> MRSTQEERFEQRIAQETAIEPQDWMPDAYRKTLIRQIGQHAHSEIVGMLPEGNWITRAPTLRRKAILLAKVQDEAGHGLYLYSAAETLGCAREDIYQKMLDGRMKYSSIFNYPTLSWADIGVIGWLVDGAAIVNQVALCRTSYGPYARAMVKICKEESFHQRQGFEACMALAQGSEAQKQMLQDAINRFWWPALMMFGPNDDNSPNSARSLTWKIKRFTNDELRQRFVDNTVPQVEMLGMTVPDPDLHFDTESGHYRFGEIDWQEFNEVINGRGICNQERLDA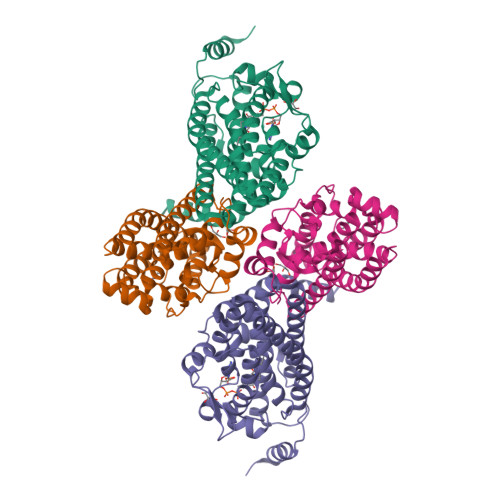KRKAWEEGTWVREAALAHAQKQHARKVA;>[2x]MGSSHHHHHHGSNQLTAYTLRLGDNCLVLSQRLGEWCGHAPELEIDLALANIGLDLLGQARNFLSYAAELAGEGDEDTLAFTRDERQFSNLLLVEQPNGNFADTIARQYFIDAWHVALFTRLMESRDPQLAAISAKAIKEARYHLRFSRGWLERLGNGTDVSGQKMQQAINKLWRFTAELFDADEIDIALSEEGIAVDPRTLRAAWEAEVFAGINEATLNVPQEQAYRTGGKKGLHTEHLGPMLAEMQYLQRVLPGQQW>MAHHHHHHMYLGLDLGTSGVKALLIDEAQNPVGAAHGELDVSRPHPGWSEQDPAQWIKACRTAIEALRAAHPKEFSAITGIGLSGQMHGATLLDAEDRVLRPCILWNDTRSYREAAELDADPAFRAITGNIVFPGFTAPKLVWVARNEADIFARIRKVLLPKDYLRLWLTGEYISDMSDSAGTSWLDTGARRWSAELLAKTGLGEGQMPQLVEGSEAAGCLRAELAAEWSLTASVIVAGGAGDNAASACGMGTVKPGHAFVSLGTSGVLFAANGAYQPKPESAVHAFCHALPRTWHQMGVILSAASALEWYSKIVGATPQSLDRELGETLKAPGSVTFLPYLSGERTPYNDAKIRGSFCGLEHEADRSALTQAVLEGVAFAIRDNLLALQSAGTEITSLTAVGGGSRSTYWLKAIATAL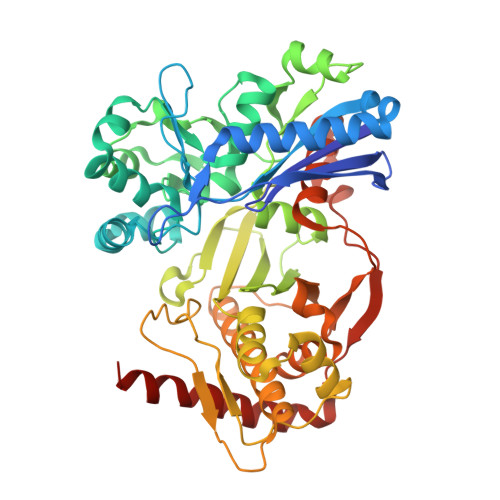NVPIALPEEGDFGAAFGAARLGLIAATGADPFTICTPPQTARTIEPEQALLSAYDEAYQRYHALYPALHALD[4x]>MASSLHSPGQAFRAALAKENPLQIVGAINANHALLAQRAGYQAIYLSGGGVAAGSLGLPDLGISTLDDVLTDIRRITDVCPLPLLVDADIGFGSSAFNVARTVKSIAKAGAAALHIEDQVGAKRCGHRPNKAIVSKEEMVDRIRAAVDARTDPNFVIMARTDALAVEGLEAALDRAQAYVDAGADMLFPEAITELSMYRRFADVAQVPILANITEFGATPLFTTDELRSAHVAMALYPLSAFRAMNRAAEKVYTVLRQEGTQKNVIDIMQTRNELYESINYYQFEEKLDALYRNKKSLEH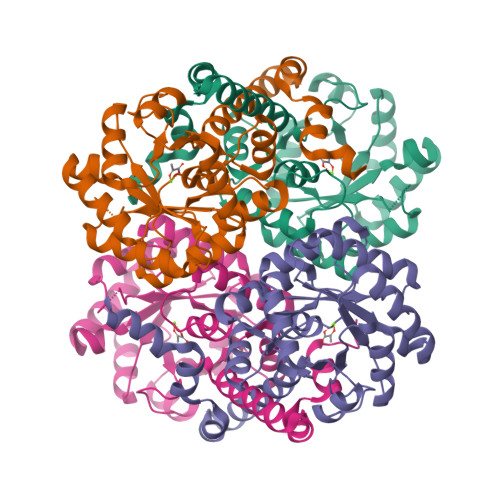HHHHH[4x]>[2x]RDQEQYIHRKCYQEFAHCYLVKYKTPQPWPNEGLIADQCPLPGLADVSFYPYQAIWDYYAKIENIRPANWTSSKLYGKARMGSYYIPKRLRNINNTHILFCSDVLYSKWYNLQNSILQNENELTKRLSNLTIGNKLKNRALPYEWAKGGLNRLFRNISVLDVCSRPEMVLLLNKTYYTFSLWEGDCNITRYNVNETVPECKDFPHRRFNDHPYSCRLWRYREGKEEVKCLTSDHTRCLYYPEY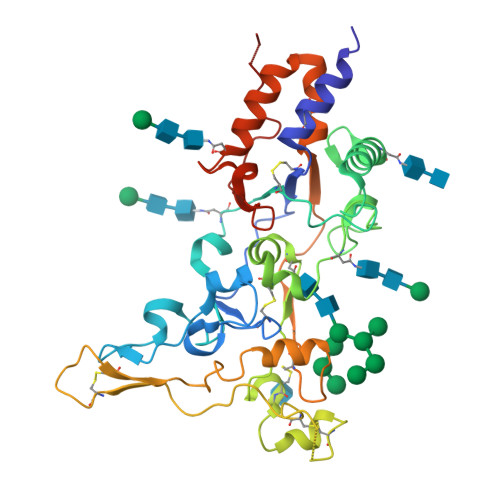SNPEALFDFGFLSYMRNFPGPQCIESTSIRQQDYEVYSIYQECKLASKTYGIDSVLFSLKNFLNYTGKPVNEMPNARAFVGLIDPKFPPTYPDDDDK> MASMTGGQQMGRDEAGITGTWY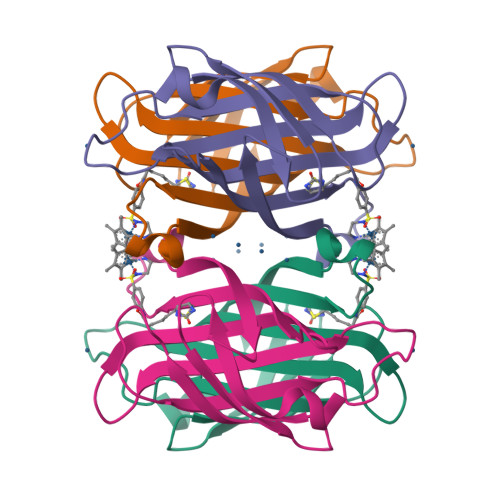NQLGSTFIVTAGADGALTGTYESAVGNAESRYVLTGRYDSAPATDGSGTALGWTVAWKNNYRNAHSATTWSGQYVGGAEARINTQWLLTAGTTEAPAWAMTLVGHDTFTKVKPSAASIDAAKKAGVNNGNPLDAVQQ In Gram-negative bacteria, conjugation is mediated by a large transport apparatus—the conjugative type IV secretion system (T4SS)—produced by the donor cell and embedded in both its outer and inner membranes. The T4SS also elaborates a long extracellular filament—the conjugative pilus—that is essential for DNA transfer. Here we present a single-particle cryo-EM structure of a T4SS complex from the R388 plasmid that comprises all four sub-complexes: OMCC, stalk, arches and IMC. Three ATPases, VirB4 (also known as TrwK), VirB11 (also known as TrwD) and VirD4, power the system.

The OMCC is composed of the O-layer embedded in the outer membrane and the I-layer located underneath within the periplasm. The O-layer, which comprises full-length VirB7 and the C-terminal domains of VirB10 (VirB10CTD) and VirB9 (VirB9CTD), and the I-layer, composed of the N-terminal domains of these proteins (termed VirB10NTD and VirB9NTD, respectively) form tetradecameric and hexadecameric assemblies, respectively. Thus, two heterodimeric VirB10NTD–VirB9NTD complexes insert into the I-layer (diametrically opposite), whereas the C-terminal domains of these two complexes are not inserted in the O-layer. As layers of pentameric VirB2 are added, the pilus grows from the bottom, pushing the VirB5 pentamer out, passing through the arches, the I-layer (no conformational changes are needed), and finally through the O-layer channel, which is known to be flexible enough to open up7,23.

>MFGRKKGDVIDAGAELERAEQERIEGEYGASELASERRPHTPGARTLLMVLLCVIAVVLVTLSYKAYKVRGVVEDDDAQPQQVVRQVIPGYTPRPIRPEPENVPEPPQPTTSVPAIQPAPVTQPVRPQPTGPREKTPYELARERMLRSGLTAGSGGGEDLPRPQGGDVPAGGLMGGGGGGGELAEKLQPMRLSGSSAGRLGNRDMLITQGTQLDCVLETRLVTTQPGMTTCHLTRDVYSTSGRVVLLDRGSKVVGFYQGGLRQGQARIFVQWSRIETPSGVVINLDSPGTGPLGEAGLGGWIDRHFWERFGGAIMISLIGDLGDWASRQGSRQGDNSIQFSNTANGVESAAAEALRNSINIPPTLYKNQGERVNILVARDLDFSDVYSLESIPTK[14x];>[14x]MKKLAIVALLASLHAVPALALDVPSSSRYDHRIRYVTYNPADVVQVDTVLGVATHIMLEEGEQYLTHAFGDSEAYAFARKGRHIFIKPQAELANTNLIVVTDRRSYKFRLQMRNDRNGAMYELAFRYPDTQARQTREANARAAVEAAFEQRVGAYYNLKYMMSGDKDIAPVNAWDDGRFTYFKFSANADLPSIYFVDAEGNESLVPRTTVGSSNNIIAVHKVNPKWMIRLGNRALAIFNEAYDPNGVPNDTGTASPAVRRVNKGGN;>MKTIIFAILMTGLLSACASAPKPKQPSDFNREPVNKTVPVEIQRGAL[14x]>PHPWFFGKIPRAKAEEMLSKQRHDGAFLIRESESAPGDFSLSVKFGNDVQHFKVLRDGAGKYFLWVVKFNSLNELVDYHRSTSVSRNQQI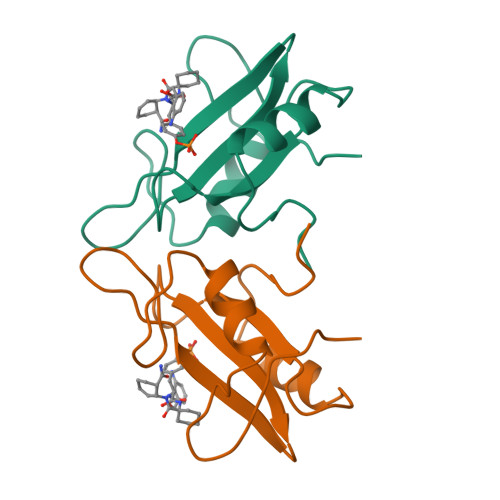FLRDIE[12x]>[2x]XSTVHEILCKLSLEGDHSTPPSAYGSVKAYTNFDAERDALNIETAIKTKGVDEVTIVNILTNRSNEQRQDIAFAYQRRTKKELASALKSALSGHLETVILGLLKTPAQYDASELKASMKGLGTDEDSLIEIICSRTNQELQEINRVYKEMYKTDLEKDIISDTSG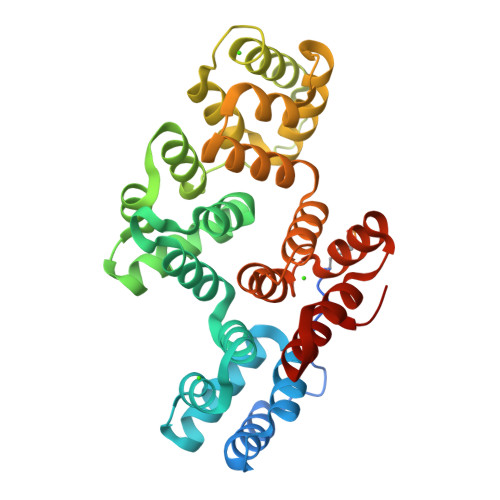DFRKLMVALAKGRRAEDGSVIDYELIDQDARDLYDAGVKRKGTDVPKWISIMTERSVPHLQKVFDRYKSYSPYDMLESIRKEVKGDLENAFLNLVQCIQNKPLYFADRLYDSMKGKGTRDKVLIRIMVSRSEVDMLKIRSEFKRKYGKSLYYYIQQDTKGDYQKALLYLCGGDD>MSDWTYSEG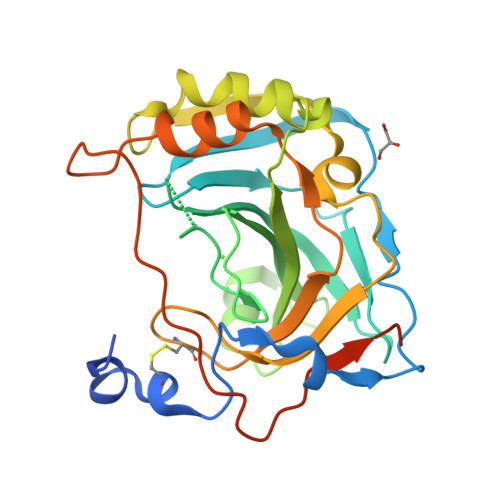ALDEAHWPQHYPACGGQRQSPINLQRTKVRYNPSLKGLNMTGYETQAGEFPMVNNGHTVQISLPSTMRMTVADGTVYIAQQMHFHWGGASSEISGSEHTVDGIRHVIEIHIVHYNSKYKSYDIAQDAPDGLAVLAAFVEVKNYPENTYYSNFISHLANIKYPGQRTTLTGLDVQDMLPRNLQHYYTYHGSLTTPPCTENVHWFVLADFVKLSRTQVWKLENSLLDHRNKTIHNDYRRTQPLNHRVVESNFPNQEYTLGSEFQAENLYFQ[2x]>TDFSNLFARDLLPAKNGEEQTVQFLLEVVDILLNYVRKTFDRSTKVLDFHHPHQLLEGMEGFNLELSDHPESLEQILVDCRDTLKYGVRTGHPRFFNQLSTGLDIIGLAGEWLTSTANTNMFTYEIAPVFVLMEQITLKKMREIVGWSSKDGDGIFSPGGAISNMYSIMAARYKYFPEVKTKGMAAVPKLVLFTSEQSHYSIKKAGAALGFGTDNVILIKCNERGKIIPADFEAKILEAKQKGYVPFYVNATAGTTVYGAFDPIQEIADICEKYNLWLHVDAAWGGGLLM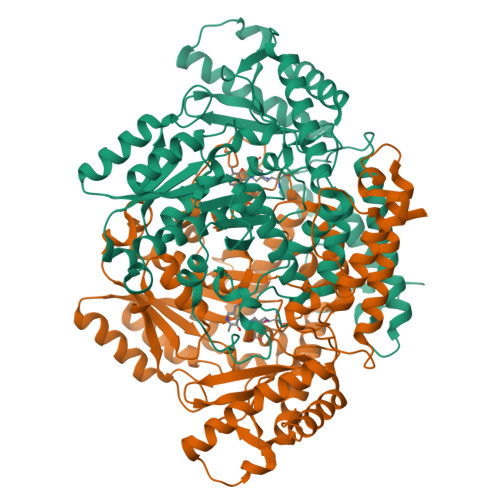SRKHRHKLNGIERANSVTWNPHKMMGVLLQCSAILVKEKGILQGCNQMCAGYLFQPDKQYDVSYDTGDKAIQCGRHVDIFKFWLMWKAKGTVGFENQINKCLELAEYLYAKIKNREEFEMVFNGEPEHTNVCFWYIPQSLRGVPDSPQRREKLHKVAPKIKALMMESGTTMVGYQPQGDKANFFRMVISNPAATQSDIDFLIEEIERLGQDLHH[2x]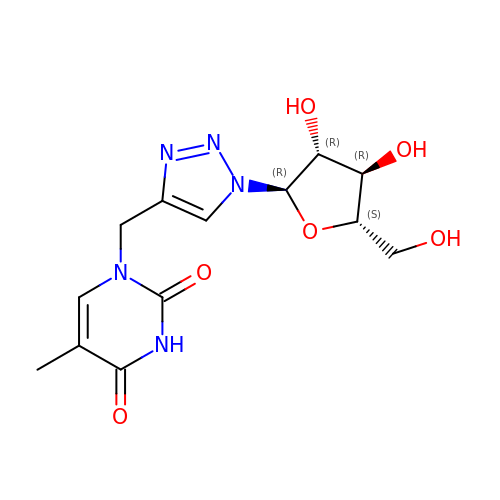1-{[1-(alpha-L-arabinofuranosyl)-1H-1,2,3-triazol-4-yl]methyl}-5-methyl-2,4-dioxo-1,2,3,4-tetrahydropyrimidine | C13 H17 N5 O6 | FVDUYFCPFLONHE-UXCLJVHYSA-N>SNAMKIAVDAMGGDNAPQAIVEGVMLAKQDFPDIEFQLYGKEAEIKKYITDEKNITIIHTDEKIASDDEPVKAIRRKKTASMVLAAQAVKNGEADAIFSAGNTGALLAAGLFIVGRIKNVERPGLMSTLPVMGEPDKGFDMLDLGANADNKPEHLVQYAVLGSFYAEKVRNVQNP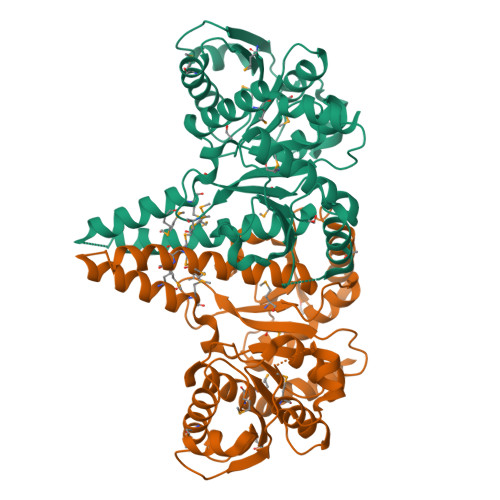RVGLLNNGTEETKGSELTKKAFELLAADETINFVGNVEARELLNGVADVVVTDGFTGNAVLKSIEGTAMNMMSLLKTAILSEGVKGKMGALLLKNALHGMKDEMDYSKHGGAVLFGLKAPVIKTHGATGPDAVRYTIRQIHTMLETQVVPQLVEYYEGKAE[2x]> TSSPSTTPINFHINKPFVFAIREKSTGVILFIGEIGEV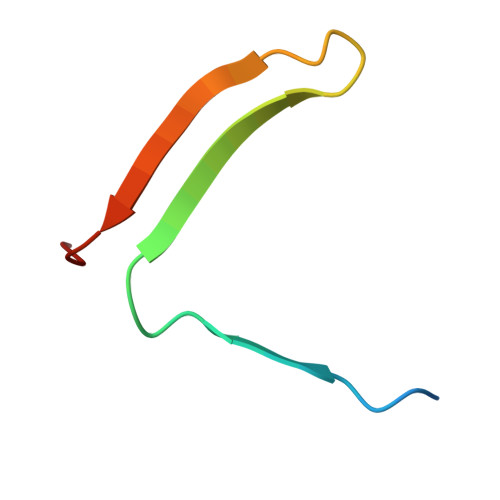KE>[2x]HHHHHHFNLPPGNYKKPKLLYCSNGGHFLRILPDGTVDGTRDRSDQ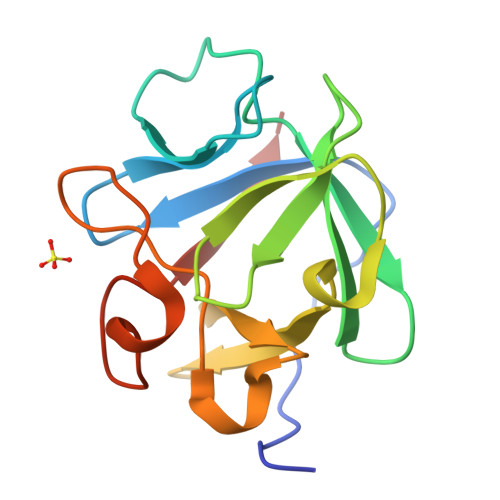HIQLQLSAESVGEVYIKSTETGQYLAMDTDGLLYGSQTPNEEALFLERLEENHYNTYISKKHAEKNWFVGLKKNGSCKRGPRTHYGQKAILFLPLPVSSD> MSHHHHHHSSGLVPRGSHMLEDLMSKEVSEEAQAHQHGKDYVDPPPAPFFDLGELKLWSFWRAAIAEFIATLLFLYITVATVIGHSKETVVCGSVGLLGIAWAFGGMIFVLVYCTAGISGGHINPAVTFGLFLARKVELLRALVYMIAQCLGAICGVGLVKAFMKGPYNQFGGGANSVALGYNKGTALGAEIIGTFVLVYTVFSATDPKRSARDSHVPILAPL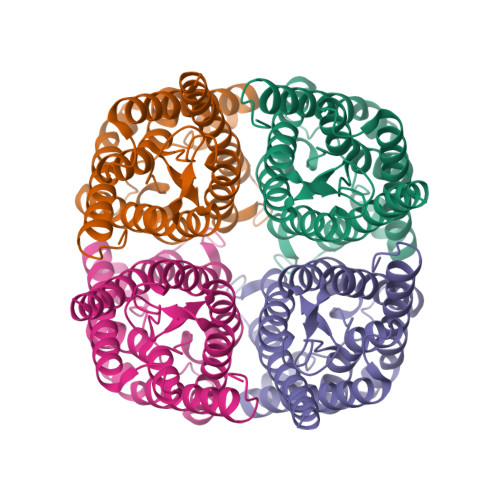PIGFAVFMVHLATIPITGTGINPARSFGAAVIFNSNKVWDDQWIFWVGPFIGAAVAAAYHQYVLRAAAIKALGEFRSNPTN> MYHRGYGGHYRGGRGGGRGHSHWHNNAPMERGGHMPSNNEGAAISSGSTGFSPLMDFFHSVEGRNYGELRSLTNETYQISENVRCTFLSIQSDPFAPGSQVRLVCPCTFSLEKVLQTTDLAAANPCRRVAAEDFILRSFHAGYRNGIPRRTSGAVQVLRPSQHVLERSTVGLVKAHQQKSGMQAEIEIFARVKLPGHGRRIDGHGAIDIFYNELVPLLEQCVVGLNEEDLHQHVICVHDQEELRSNLLGAGYVAFVANGAILPRDAGNSDKPLRDNAVPFQSPKSLECSFTLPHSGKTITGMGLPPGLTLIAGGGFHGKSTLLRALEVGIYNHVPDDGRTYVVVDPTAVKIRAEDRRSVHGVDISPFINNLPFGKTTNFFVTADASGSTSQAANIMEALELGSQLLLLDEDTCATNLMYRDALMQMLVPRAQEPITPFVERVADLSQNHGVSSIMVIGGSGQYFPQARVVLVMNAYQISDCTKEAKEIASNSSLPALNPPGDTASVFIPDVNRCFDPDGSFTTVRRRRGREGTKVSGIGTESIRFSEETIDLSMVEQIVEEGQVNAIAQCLALLYDGEPRIVPEMTTKGGALTQLPSPGGVCEIQRGKFNSNFSSMIAGCCSHQHDKRLELRTPSCYLPRGFTSATRHIEIGAALNRLRTLRTVTAKR

One such protein, MRB1590, was originally identified in MRB1 complexes immunoprecipitated or tandem affinity purified with GAP1/GAP2 (21). In vivo experiments suggest that MRB1590 effects editing of several mitochondrial mRNA transcripts, in particular that encoding subunit 6 of ATPase synthase (A6). Structural studies showed that MRB1590 contains an ABC-like ATPase domain, which is embedded between N- and C-terminal domains that harbor novel folds. We show that residues in the basic N-terminal domain are involved in RNA binding and crystal structures capturing open and closed states of MRB1590 suggest possible mechanisms for how this protein may participate in RNA editing processes.

Hence, to gain insight into its function at the molecular level, we determined its crystal structure by single wavelength anomalous diffraction (SAD). The structure was refined to final Rwork/Rfree values of 20.4%/26.2% to 2.6 Å resolution. Although the full length protein was crystallized, N-terminal residues 1–51 were not visible. The MRB1590 structure revealed the presence of an expansive dimer that buries 2373 Å2 of subunit surface from solvent. MRB1590 dimerization is mediated primarily by residues located in the central and C-domains of the protein and juxtaposes the two N-domains of the dimer together, creating a pore or cleft between them. In fact, although no nucleotide was added to MRB1590 prior to crystallization, electron density for an ADP molecule was found in this central domain. As noted, although no nucleotide was provided in the crystallization setups, an ADP molecule was found in the structure. These data suggest that MRB1590 function is likely tied to adenine nucleotide binding. In fact, there are direct contacts between residues in the N-domains in the closed state. Specifically, the two-fold related Phe95 side chains stack together as do the side chains of Arg199. In addition, the Arg199 side chains make hydrogen bonds to Asn65’.> MSGDENPASKPTPVQDVQGDGRWMSLHH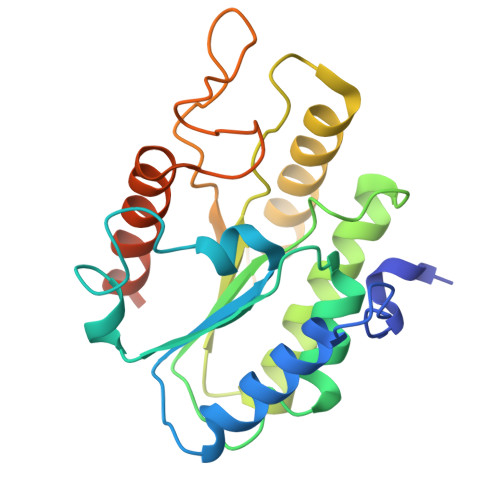RFVADSKDKEPEVVFIGDSLVQLMHQCEIWRELFSPLHALNFGIGGDSTQHVLWRLENGELEHIRPKIVVVWVGTNNHGHTAEQVTGGIKAIVQLVNERQPQARVVVLGLLPRGQHPNPLREKNRRVNELVRAALAGHPRAHFLDADPGFVHSDGTISHHDMYDYLHLSRLGYTPVCRALHSLLLRLLTQDQGQGGAPLPEPSP> MFNRTTQLKSKHPCSVCTRRKVKCDRMIPCGNCRKRGQDSECMKSTKLITASSSKEYLPDLLLFWQNYEYWITNIGLYKTKQRDLTRTPANLDTDTEECMFWMNYLQKDQSFQLMNFAMENLGALYFGSIGDISELYLRVEQYWDRRADKNHSVDGKYWDALIWSVFTMCIYYMPVEKLAEIFSVYPLHEYLGSNKRLNWEDGMQLVMCQNFARCSLFQLKQCDFMAHPDIRLVQAYLILATTTFPYDEPLLANSLLTQCIHTFKNFHVDDFRPLLNDDPVESIAKVTLGRIFYRLCGCDYLQSGPRKPIALHTEVSSLLQHAAYLQDLPNVDVYREENSTEVLYWKIISLDRDLDQYLNKSSKPPLKTLDAIRRELDIFQYKVDSLEEDFRSNNSRFQKFIALFQISTVSWKLFKMYLIYYDTADSLLKVIHYSKVIISLIVNNFHAKSEFFNRHPMVMQTITRVVSFISFYQIFVESAAVKQLLVDLTELTANLPTIFGSKLDKLVYLTERLSKLKLLWDKVQLLDSGDSFYHPVFKILQNDIKIIELKNDEMFSLIKGLGSLVPLNKLRQESLL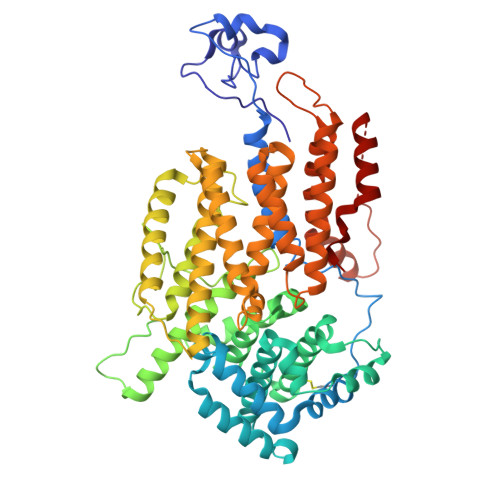EEEDENNTEPSDFRTIVEEFQSEYNISDILS1-(2,5-DIOXO-2,5-DIHYDRO-1H-IMIDAZOL-4-YL)UREA | C4 H4 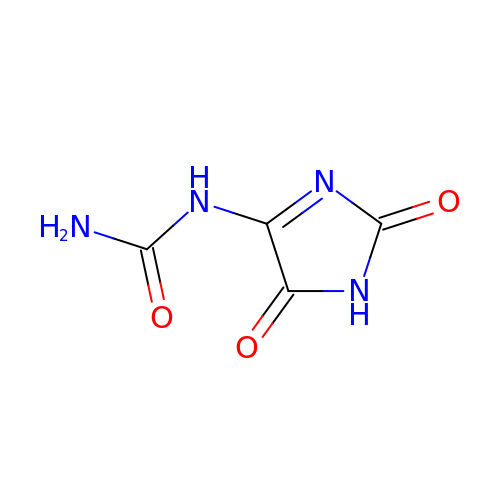N4 O3 | MFAONEQLPARJAO-UHFFFAOYSA-N> GKKAWCWASYLEEEKAVAVPAKLFKEHQSFPYNKNGFKVGMKLEGVDPEHQSVYCVLTVAEVCGYRIKLHFDGYSDCYDFWVNADALDIHPVGWCEKTGHKLHPPKGYKEEEFNWQTYLKTCKAQAAPKSLFENQNITVIPSGFRVGMKLEAVDKKNPSFICVATVTDMVDNRFLVHFDNWDESYDYWCEASSPHIHPVGWCKEHRRTLITPPGYPNVKHFSWDKYLEETNSLPAPARAFKVKPPHGFQKKMKLEVVDKRNPMFIRVATVADTDDH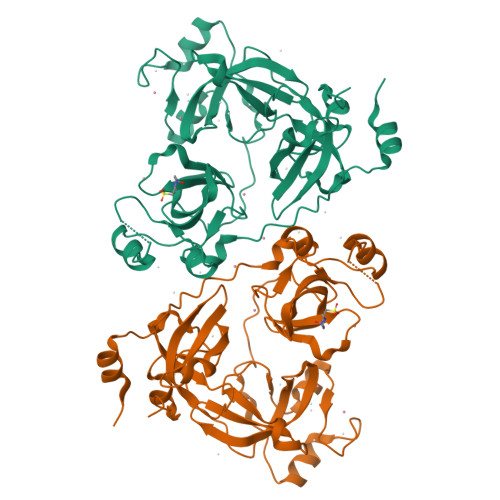RVKVHFDGWNNCYDYWIDADSPDIHPVGWCSKTGHPLQPPLSPLELME>[8x]LMPTERIDINEREDCTASEMTAPTVPVALVTGAAKRLGRSIAEGLHAEGYAVCLHYHRSAAEANALSATLNARRPNSAITVQADLSNVATAPVSGADGSAPVTLFTRCAELVAACYTHWGRCDVLVNNASSFYPTPLLRNDEDGH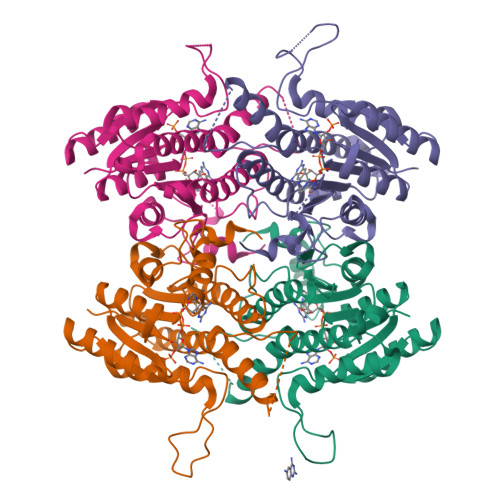EPCVGDREAMETATADLFGSNAIAPYFLIKAFAHRVAGTPAKHRGTNYSIINMVDAMTNQPLLGYTIYTMAKGALEGLTRSAALELAPLQIRVNGVGPGLSVLVDDMPPAVWEGHRSKVPLYQRDSSAAEVSDVVIFLCSSKAKYITGTCVKVDGGYSLTRA beta-D-fucopyranose 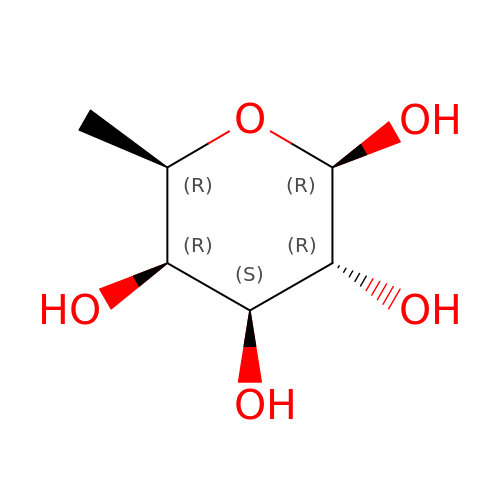| C6 H12 O5 | SHZGCJCMOBCMKK-FPRJBGLDSA-N1-[(2R,15R)-2-[(1-amino-4-fluoroisoquinolin-6-yl)amino]-4,15,17-trimethyl-3,12-dioxo-13-oxa-4,11-diazatricyclo[14.2.2.1~6,10~]henicosa-1(18),6(21),7,9,16,19-hexaen-7-yl]cyclobutane-1-carboxylic 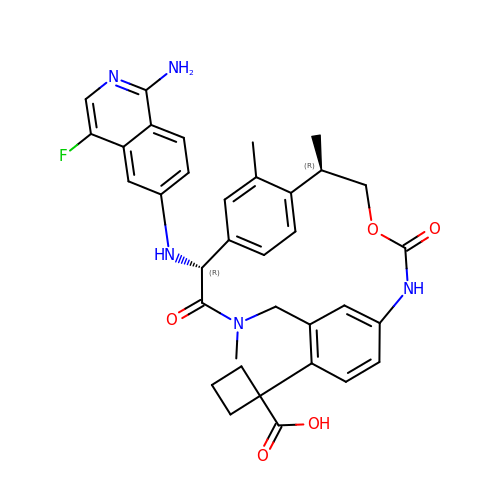acid | C35 H36 F N5 O5 | PROYMPSAMYSXNO-WENCNXQZSA-N> MGQNITARIGEPLVLSCKGAPKKPPQQLEWKLNTGRTEAWKVLS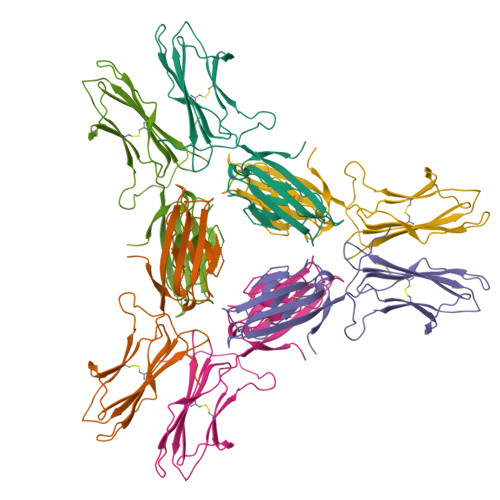PQGGPWDSVARILPNGSLLLPATGIVDEGTFRCRATNRRGKEVKSNYRVRVYQIPGKPEIVDPASELTASVPNKVGTCVSEGSYPAGTLSWHLDGKLLIPDGKETLVKEETRRHPETGLFTLRSELTVIPTQGGTHPTFSCSFSLGLPRRRPLNTAPIQLRVREP> MSSQIRQNYSTDVEAAVNSLVNLYLQASYTYLSLGFYFDRDDVALEGVSHFFRELAEEKREGYER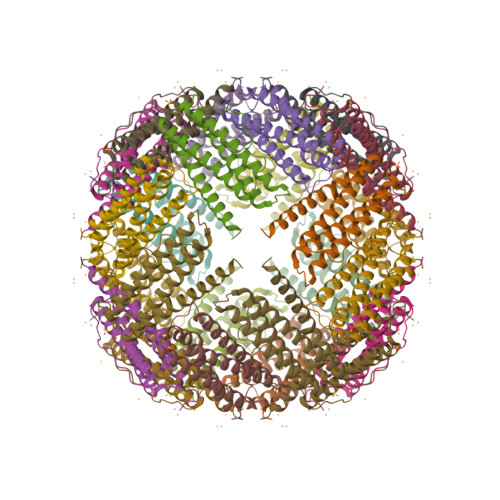LLKMQNQRGGRALFQDIKKPAEDEWGKTPDAMKAAMALEKKLNQALLDLHALGSARTDPHLCDFLETHFLDEEVKLIKKMGDHLTNLHRLGGPEAGLGEYLSSKGSLSSTTKSLLSPATSEGPLAK> GSHMNNDFNGKITLAITGASGASYAMRLIECLIAANYQLYILCSSAGRISLDTEVGVKIPSSPDAASKFLTEKYQAKDQQITVFGKEQWFSPVASGSSAPKQMVVCPCSTGTMAAICHGMSDNLIERAADVVIKERGQLILMVRETPFSTLHLQNMLSLSQQGVTIMPASPGFYHKVETIEDLIDFMVGRVLDHLGIEQDIMPRWGYNI

In prokaryotic organisms, several ubi gene clusters encoding a set of enzymes (UbiA, UbiB, UbiC, UbiD, UbiE, UbiF, UbiG, UbiH, and UbiX) produce ubiquinone from its precursor, chorismate. The monomer structure adopts a typical Rossmann-fold topology comprising eight α-helices (residues 19–32, 42–52, 60–71, 89–91, 107–115, 121–132, 147–159, and 177–192) and six β-strands (residues 8–13, 35–40, 78–81, 99–103, 135–140, and 162–165). The crystallographic symmetries of both crystal structures generate spherical dodecamers with dimensions of 105 Å × 93 Å × 95 Å. The monomeric structure of CpsUbiX is stabilized by two different patches of inter-subunit contacts, namely patches 1 and 2, to generate a dodecamer.

Moreover, a V47S mutation resulted in complete loss of FMN binding, allowing us to produce an FMN-free form of CpsUbiX without affecting overall structure of the protein. Here, we confirmed that electron density corresponding to FMN was absent in the crystal structure of the V47S mutant. Val47 is located on the α2 helix, which extends from the β2 strand of the central β-sheet and makes van der Waals interactions with the dimethyl phenyl moiety of isoalloxazine. Therefore, mutating the Val47 to Ser significantly affected this hydrophobic interaction, resulting in the mutant protein having a low affinity toward FMN. FMN-bound CpsUbiX crystallized in the orthorhombic space group (C2221) with 6 monomers in the asymmetric unit, while FMN-free CpsUbiX crystallized in the cubic space group (P23) with one molecule in the asymmetric unit. The phosphate-binding site in FMN-free UbiX is occupied by a sulfate ion (SO4 II). On the other hand, the C-terminus is parallel to α7 in FMN-free CpsUbiX and is stabilized by Met199 and Trp202 through hydrophobic and hydrogen bond interactions. Tyr204 is exposed to the bulk solvent in the FMN-free CpsUbiX. In contrast to the FMN-bound CpsUbiX, the structure of the C-terminal region of the FMN-free CpsUbiX extends into a β-sheet region of the core domain with the conformational difference starting at the Glu195 residue. Loss of this interaction in FMN-free CpsUbiX causes the residues His172 to Val174 to be relaxed and the Phe170–Thr176 loop region to drift towards the neighboring molecule. This in turn leads to the formation of a large solvent channel connected to the putative active site in the FMN-free form.>GPMANSSVELRVAEAYPEDVGRGIVRMDKQTRAKLGVSVG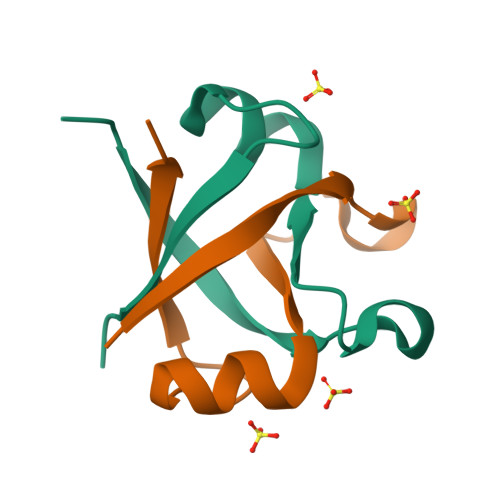DYVEVKKVD[4x]>[6x]GSTRVDWKETPEAHVFKADLPGLKKEEVKVE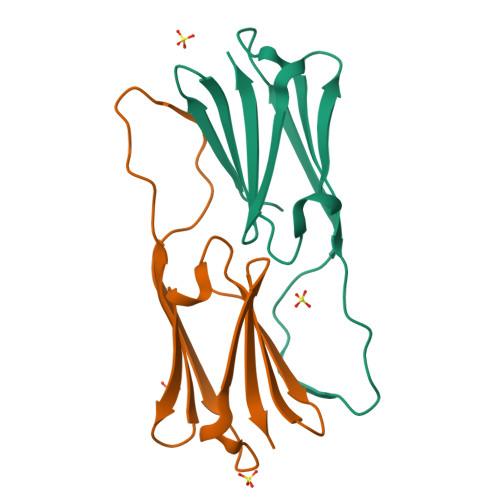VEDDRVLQISGERSVEKEDKNDEWHRVERSSGKFLRRFRLPENAKMDKVKASMENGVLTVTVPK>SVDVGDYRVNSITAQVIPQSQIVMSGDTYKANIVLSSVDTTQRPDVFVNGKLLSPENMGLFTATAGAPGTYPVKGYIEMMGNDGVKIRRDFESEYFVTEPMASVAPTMMNVLYAGIDNPINIAVPGVAQQNVSATINNGTLTRRGNLWI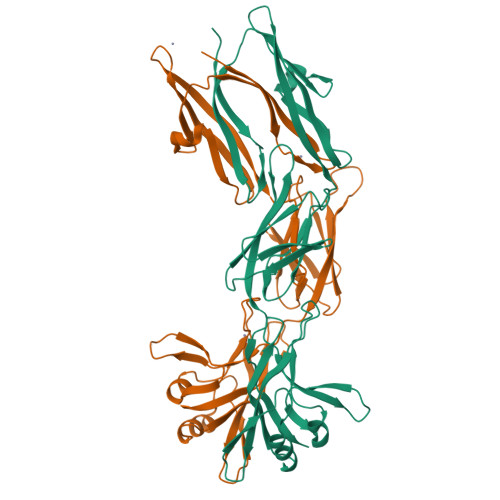ARPTKVGSEAIISVTAQSGGRTIQMAKTTLRVRALPDPLPYIEYKDVQGNTKRFKGGRLGKREILAAGGIKAALDDDLLEVNYTVVKFQLVFYDSMGNSIPEVSDGASFSERQKRQIQNLGKGKRFYVTEVIARGPDGIERKIPAIEVIVN[2x]> PF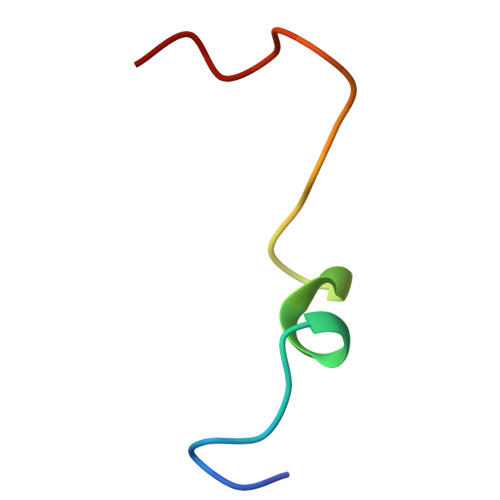DQMTIEDLNEVFPETKLDKKKY> MDYKDDDDKENLYFQGATVTATTKVPEIRDVTRIERIGAHSHIRGLGLDDALEPRQASQGMVGQLAARRAAGVVLEMIREGKIAGRAVLIAGQPGTGKTAIAMGMAQALGPDTPFTAIAGSEIFSLEMSKTEALTQAFRRSIGVRIKEGPPGVVHTVSLHEIDVINSRTQGFLALFSGDTGEIKSEVREQINAKVAEWREEGKAEIIPGVLFIDEVHMLDIESFSFLNRALESDMAPVLIMATNRGITRIRGTSYQSPHGIPIDLLDRLLIVSTTPYSEKDTKQILRIRCEEEDVEMSEDAYTVLTRIGLETSLRYAIQ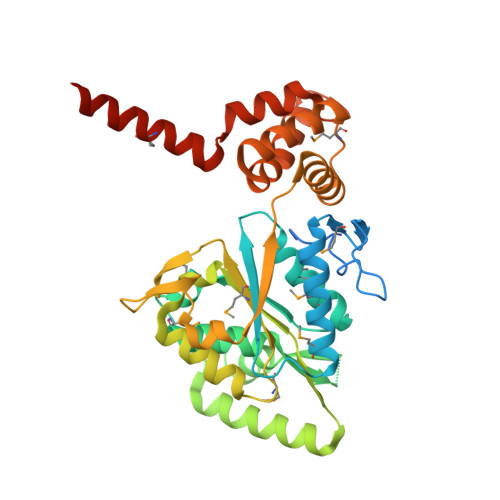LITAASLVCRKRKGTEVQVDDIKRVYSLFLDESRSTQYMKEYQDAFLFNELKGETMDTS(2S)-(3,5-difluorophenyl)(hydroxy)acetic acid | C8 H6 F2 O3 | 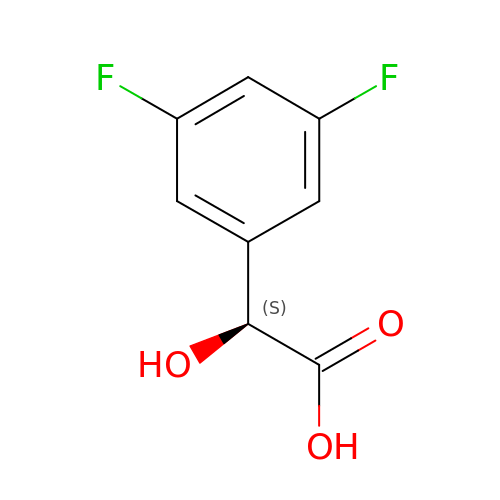PHMLPPFFMSRWBK-ZETCQYMHSA-N>GRFNPFIHQQDVYVQIDRDGRHLSPGGTEYTLDGYNASGKKEEVTFFAGKELRKNAYLKVKAKGKYVETWEEVKFEDM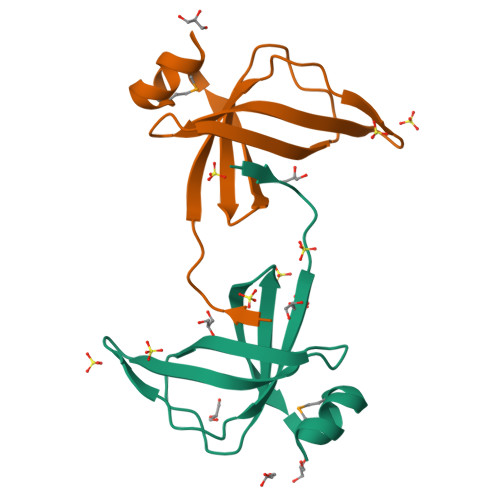PDSVQSKLK[2x]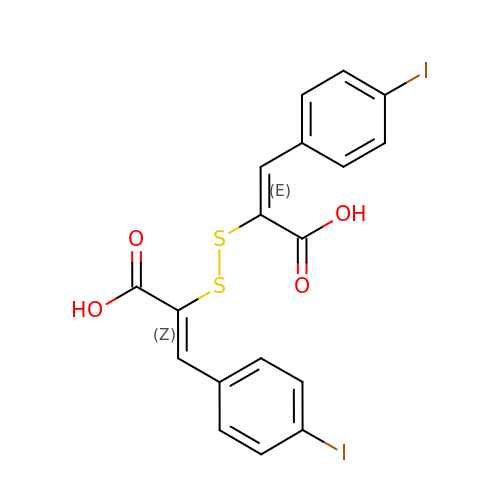(2E,2'Z)-2,2'-disulfanediylbis[3-(4-iodophenyl)prop-2-enoic acid] | C18 H12 I2 O4 S2 | RLKZEUBAGNQDNM-CKOAPEAFSA-N> QIGWRREGIKYRRNELFLDVLESVNLLMSPQGQVLSAHVSGRVVMKSYLSGMPECKFGMNDKIVIEX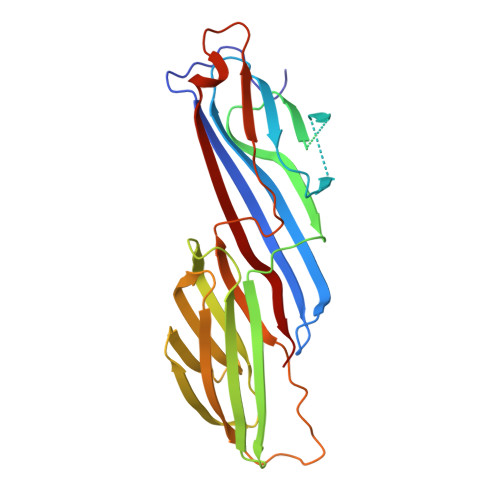XXXXXXXXXXXXXXXXXXXXXXXXXXXXXXXXXXXXRSISFIPPDGEFELMRYRTTKDIILPFRVIPLVREVGRTKLEVKVVIKSNFKPSLLAQKIEVRIPTPLNTSGVQVICMKGKAKYKASENAIVWKIKRMAGMKESQISAEIELLPTNDKKKWARPPISMNFEVPFAPSGLKVRYLKVFEPKLNYSDHDVIKWVRYIGRSGIYETRC Mechanosensitive (MS) ion channels are a ubiquitous type of molecular force sensor sensing forces from the surrounding bilayer. Here we determine the structures of plant and mammalian OSCA/TMEM63 proteins, allowing us to identify essential elements for mechanotransduction and propose roles for putative bound lipids in OSCA/TMEM63 mechanosensation. Briefly, the central cavity created by the dimer interface couples each subunit and modulates dimeric OSCA/TMEM63 channel mechanosensitivity through the modulating lipids while the cytosolic side of the pore is gated by a plug lipid that prevents the ion permeation.

Then we solved the AtOSCA1.1 channel structure in the lipid nanodisc environment at 2.5 Å resolution. The 2.5 Å resolution map allowed us to build the model of nearly full-length AtOSCA1.1. We used the parallelogram of the midpoint of the transmembrane segments of AtOSCA1.1 to represent the central cavity area, specifically the Cα atoms of the F384 and I660 residues. This illustrated that the area of the central cavity was extended. We found a strong lipid density on the extracellular side of the central cavity and a lyso-lipid-like molecule fitted this density well. The putative lyso-lipids seem to insert into the central cavity and extend the central cavity like a rivet docking in the huge lipid storage cavity, thus resulting in the extension of the lipid storage cavity and allosterically regulating M6 resulting in channel activation, which is consistent with our previous electrophysiological finding that lyso-lipids promote OSCA channel activation. As the putative lyso-lipid in the central cavity may regulate the channel activity, we refer to it as a ‘modulating’ lipid. The mutation of H651A (a putative lyso-lipid coordinating residue) right shifts the pressure response curve indicative of a channel less sensitive to mechanical force. The addition of calcium at the dimeric interface of TMEM16A is reminiscent of the putative lyso-lipid in the central cavity of the dimeric AtOSCA1.1 channel.

>[2x]MATLKDIGVSAGINILTAFIFFIIFAFLRLQPFNDRVYFSKWYLRGLRSSPASGGGFAGRFVNLELRSYLKFLHWMPEALKMPERELIDHAGLDSVVYLRIYWLGLKIFAPIAMLAWAVLVPVNWTNNELELAKHFKNVTSSDIDKLTISNIPEGSNRFWAHIIMAYAFTIWTCYMLMKEYETVANMRLQFLASEGRRPDQFTVLVRNVPPDPDETVSELVEHFFLVNHPDNYLTHQVVCNANKLADLVSKKTKLQNWLDYYQLKYTRNNSQIRPITKLGCLGLCGQKVDAIEHYIAEVDKTSKEIAEERENVVNDQKSVMPASFVSFKTRWAAAVCAQTTQTRNPTEWLTEWAAEPRDIYWPNLAIPYVSLTVRRLVMNVAFFFLTFFFIIPIAFVQSLATIEGIEKVAPFLKVIIEKDFIKSLIQGLLAGIALKLFLIFLPAILMTMSKFEGFTSVSFLERRSASRYYIFNLVNVFLGSVIAGAAFEQLNSFLNQSPNQIPKTIGMAIPMKATFFITYIMVDGWAGVAGEILMLKPLIIYHLKNAFLVKTEKDREEAMNPGSIGFNTGEPQIQLYFLLGLVYAPVTPMLLPFILVFFALAYVVYRHQIINVYNQEYESAAAFWPDVHGRVITALIISQLLLMGLLGTKHAASAAPFLIALPVITIGFHRFCKGRFEPAFVRYPLQEAMMKDTLERAREPNLNLKGYLQDAYIHPVFKGGDNDDDGDMIGKLENEVIIVPTKRQSRRNTPAPSRISGESSPSLAVINGKEV>[3x]ADGQQGAPLNSPNTYDVTTWRIKAHPEVTAQSDIGAVINDIIADIKQRQTSPDARPGAAIIIPPGDYDLHTQVVVDVSYLTIAGFGHGFFSRSILDNSNPTGWQNLQPGASHIRVLTSPSAPQAFLVKRAGDPRLSG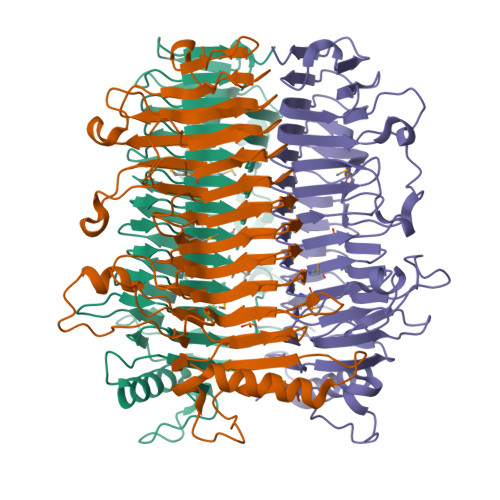IVFRDFCLDGVGFTPGKNSYHNGKTGIEVASDNDSFHITGMGFVYLEHALIVRGADALRVNDNMIAECGNCVELTGAGQATIVSGNHMGAGPDGVTLLAENHEGLLVTGNNLFPRGRSLIEFTGCNRCSVTSNRLQGFYPGMLRLLNGCKENLITANHIRRTNEGYPPFIGRGNGLDDLYGVVHIAGDNNLISDNLFAYNVPPANIAPAGAQPTQILIAGGDANVVALNHVVSDVASQHVVLDASTTHSKVLDSGTASQITSYSSDTAIRPTP> ENDNAPLFTRPVYEVSVRENNPPGAYLATVAARDRDLGRNGQVTYRLLEAEVGRAGGAVSTYVSVDPATGAIYALRSFDYETLRQLDVRIQASDGGSPQLSSSALVQVRVLDQNDHAPVLVHPAPANGSLEVAVPGRTAKDTVVARVQARDADEGANGELAFELQQQEPREAF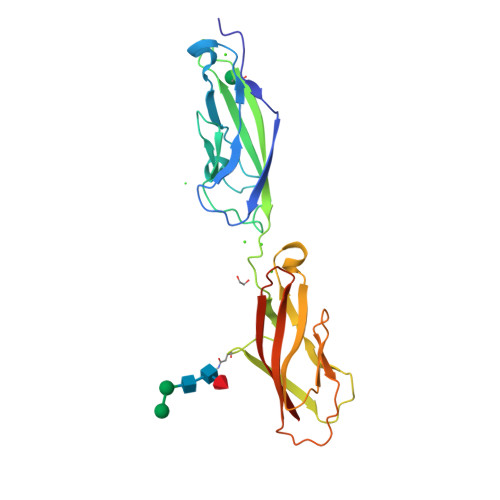AIGRRTGEILLTGDLSQEPPGRVFRALLVISDGGRPPLTTTATVSFVVTAHHHHHH>MEQRITLKDYAMRFGQTKTAKDLGVYQSAINKAIHAGRKIFLTINADGSVYAEE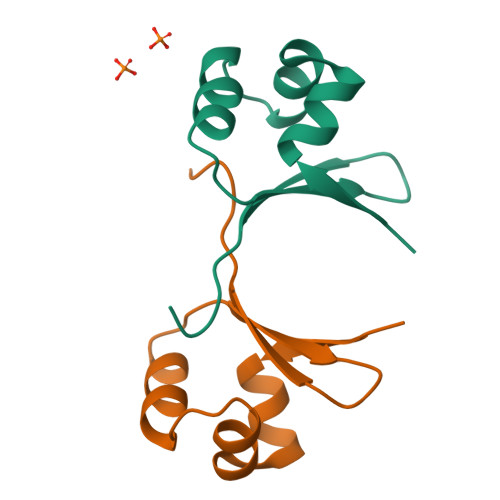VKPFPSNKKTTA[4x]>[2x]SDPVDYQAEDATIVQG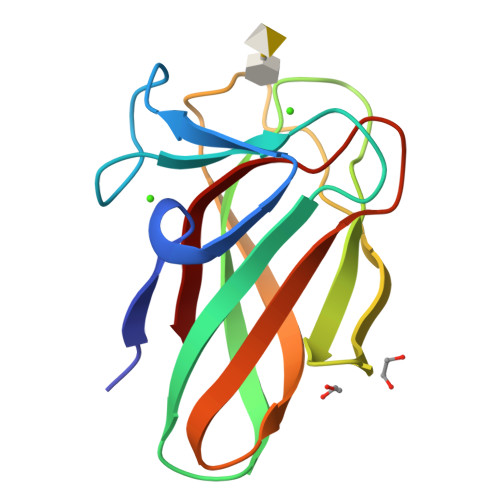AVESNHAGYTGTGFVNYDNVAGSSVEWTVTVPSAGTYDVVVRYANGTTTSRPLDFSVNGSISASGVAFGSTGTWPAWTTKTVRVTLAAGVNKIKAVATTANGGPNVDKITL> MPSNNRYDVTEWPAGNPAKDIGEVINSIIADIKARQGAADVDDGGKPGAVIYLPPGDYHLRTQVLIDISFLRIEGSGHGFTSSSIRFNVPEEEWPDLHELWPGGSRVIVDLPAGGAGDSAAGAAFLVAREGSPRISSVEFSNFCIDGLHFTADGSGRHPENTYANGKTGIHVASANDSFRVTDMGFVYLENALTIHKADALSIHHNFIAECGSCIELRGWGQASKITDNLVGAGPRGHSIYAENHGGLLVT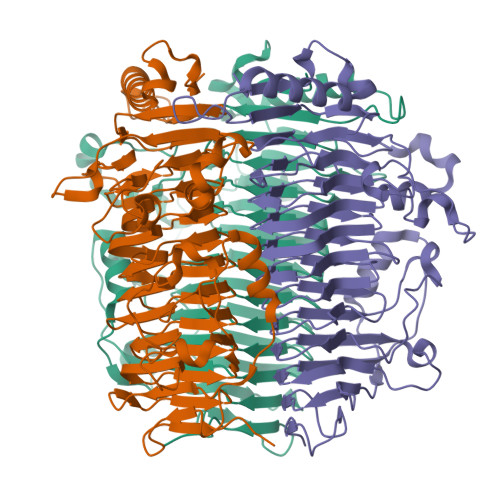ANNVFPRGASSVHFKGVTRSSVTNNRLHAFYPGMVRLEENSSENLVATNHFLRDHEPWTPFFGVDNGLDDLTGLLSISGNNNSVIGNHFSEVVDANEIRPEGATPVIIRLTAGTGNFVSTNHVVAMDVDAASSDSCFEAQVDALLATEAADLAVTAVLVDPGSARNTILDSGSDTQVVADRAVNAIRATPTVGF The housekeeping enzyme glucose 6-phosphate dehydrogenase (G6PD) (EC 1.1.1.49) is the first and rate-limiting enzyme of the PPP. It catalyzes the oxidation of glucose 6-phosphate (G6P) originating from glycolysis to 6-phospho-D-glucono-1,5-lactone (6PL), whereby the cofactor NADP+ is reduced to NADPH. In the present study, we describe the crystal structures of Leishmania donovani G6PD (LdG6PD), both native and complexed with one or both substrates. The LdG6PD monomer contains three domains: an N-domain (Q5-K49), the NADP+ binding “Rossmann-like” domain (residues D50-I248), and a β + α domain (residues D249-K552).

We observed conformational changes compared to the apo structure due to G6P binding alone. Within the G6P binding pocket, this conformational change was mainly visible through Y251 and surrounding residues (H250-Y254). Significantly larger conformational changes than in the structures complexed with NADP(H) are observed after binding substrate G6P. Moreover, the angle between the “Rossmann-like” domain and the β + α domain is reduced when G6P is bound. Structural comparison of the monomers shows that regions I248–I260 (α9) and P481–F499 (α14) rearrange, with the main chain atoms shifting by about 1.5 Å and the Y251 side chain by about 3 Å. Furthermore, residues H250, K254, M256 (α9), H312 (α12), and Y484 (α14) adopt different side-chain conformations. Remarkably in all structures, G6P is bound only in subunit B of the G6PD dimer, although subunits A and B are essentially similar (RMSD ~ 0.7 Å). However, in G6P-bound LdG6PD structures, the position of G6P that best explains the electron density is different from that of homologous G6PD structures. Compared to these structures, the G6P conformation is rotated by 180° and located in a cleft, formed by amino acids D482-A483, Q440, H250-Y251, and K254. Finally, we interpret the G6P-induced shift, leading to a 45° rotation of the N-domain and a decreased angle between the β-α domain and the “Rossmann-like” domain, as a conformational change towards the catalytic form.

>MSEEQSHADQDAYVADVDGILDVLRAQVLERKPDDIFQFISKSALSLQKDRGAESCDRINCKVKDEQKSRALTIIVFGASGDLAKKKTFPALFDLYCGGLLPPEVNIIGYARTKVDDVEKWKHETLMKYFSNLSERGCHAEDFLKHISYFCGAYDSVDDFKRLDAVIREKENAFKGPEKGGNRLFYLALPPSVFASVCESIHKGAMPQEVGGWVRVIIEKPFGRDTKSSAELSQALEPFFDESQLYRIDHYLGKEMVQNIITTRFANRIFSAVWNASNIACVQITFKETIGTEGRGGYFDNIGIIRDVMQNHLTQILALLAMEKPRSLDAECIRDEKVSVLKCIEPITKENCVLGQYTASADGSIPGYLEDVTVPEGSTCPTFAVMRLNINNDRWAGVPFILKAGKAVEQKYVAIRIQFRDEVHPYGEATQRNELVIRAQPSEAMYVKITTKVPGLSGDLRQTHQTELDLTYHTRYDVRLPDAYESLINDALLGNSTNFVRKDELDVAWRIFTPLLHQIDSGEIKPIPYQAGTRGPKEADEFIANNGFKHQKGYHWLPSNKL[2x]beta-D-arabinofuranose 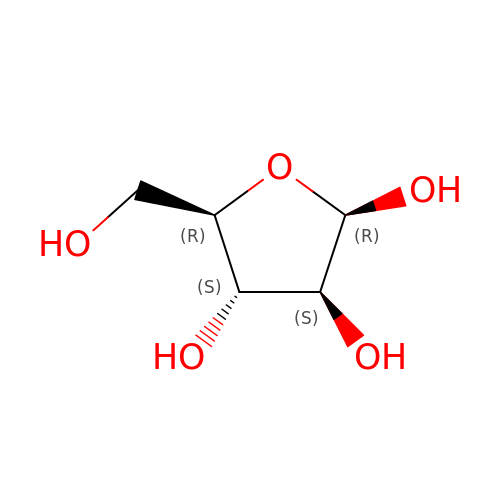| C5 H10 O5 | HMFHBZSHGGEWLO-SQOUGZDYSA-N>GAPPAPALRIDYPKALQILTEGGTHMVCTGRTHTDRLCRFKWLCYSSEAE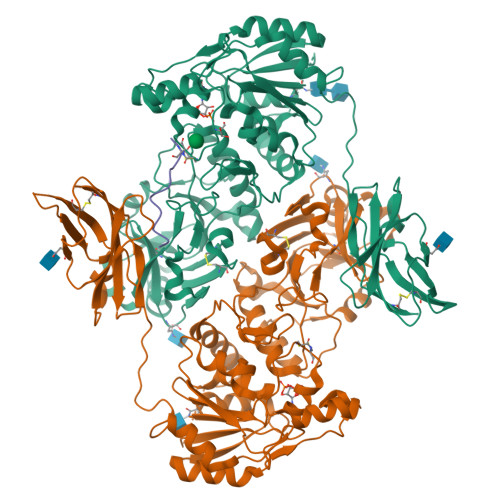EFIFFHGNASVMLPSLGSRRFQPALLDLSTVEDHNTQYFNFVELPAAALRFMPKPVFVPDVALIANRFNPDNLMHVFHDDLLPLFYTLRQFPGLAREARLFFMEGWGEGAHFDLYKLLSPKQPLLRAQLKALGRLLCFSHAFVGLSKVTTWYQYGFVQPQGPKANILVSGNEIRQFAHFLMEKLNVSQAGGPLGEEYILVFSRTQNRLILNEAELLLALAQEFQMKTVTVSLEDHAFADVVRLVSNASMLVSMHGAQLVTALFLPRGAAVVELFPYAVNPDHYTPYKTLATLPGMDLQYIAWQNTMPENTVTHPERPWDQGGIAHLDRAEQARILQSREVPRHLCCRNPEWLFRIYQDTKVDIPSLIQTIRRVVKGHPGPRKQKWTVSLYPGKVREARCQASVQGASEARLSVSWQIPWNLKYLKVREVKYEVWLQEQGENTYVPYMLALQNHTFTENIKPFTTYLVWIRCIFNKTLLGPFADVLVCST[2x];> XQTPTLGPIQPTRX>[2x]DVSGSLRIAIPVSFSQELIANLCSGFMRLYPNVELDVQFTDND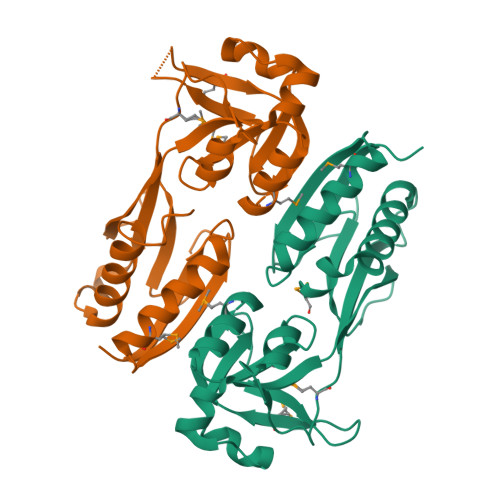IGLVGEGYDIAIKYGPLQSSDLVARLLFERQPILVASPGYLKTRGTPATPKELSDHSGILLGTSRSAPIWPLGKGTRKTMVSFQRKVRVNSPIMVKQLALDDFGIAMLSNSACKTELANGQLVPILQEWPMEPFKVYGVYSSRRQLATNISAFLDFFVKRFSSQESLQSLM>MRGCLRLALLCALPWLLLAASPGHPAKSPRQPPAPRRDPFDAARGADFDHVYSGVVNLSTENIYSFNYTSQPDQVTAVRVYVNSSSENLNYPVLVVVRQQKEVLSWQVPLLFQGLYQRSYNYQEVSRTLCPSEATNETGPLQQLIFVDVASMAPLGAQYKLLVTKLKHFQLRTNVAFHFTASPSQPQYFLYKFPKDVDSVIIKVVSEMAYPCSVVSVQNIMCPVYDLDHNVEFNGVYQSMTKKAAITLQKKDFPGEQFFVVFVIKPEDYACGGSFFIQEKENQTWNLQRKKNLEVTIVPSIKESVYVKSSLFSVFIFLSFYLGCLLVGFVHYLRFQRKSIDGSFGSNDGSGNMVASHPIAASTPEGSNYGTIDESSSSPGRQMSSSDGGPPGQSDTDSSVEESDFDTMPDIESDKNIIRTKMFLYLSDLSRKDRRIVSKKYKIYFWNIITIAVFYALPVIQLVITYQTVVNVTGNQDICYYNFLCAHPLGVLSAFNNILSNLGHVLLGFLFLLIVLRRDILHRRALEAKDIFAVEYGIPKHFGLFYAMGIALMMEGVLSACYHVCPNYSNFQFDTSFMYMIAGLCMLKLYQTRHPDINASAYSAYASFAVVIMVTVLGVVFGKNDVWFWVIFSAIHVLASLALSTQIYYMGRFKIDLGIFRRAAMVFYTDCIQQCSRPLYMDRMVLLVVGNLVNWSFALFGLIYRPRDFASYMLGIFICNLLLYLAFYIIMKLRSSEKVLPVPLFCIVATAVMWAAALYFFFQNLSSWEGTPAESREKNRECILLDFFDDHDIWHFLSATALFFSFLVLLTLDDDLDVVRRDQIPVFENLYFQGDYKDDDDKHHHHHHHH[2x]

Two mammalian homologs of systemic RNA interference defective protein 1 (SID-1) (SIDT1/2) are suggested to function as double-stranded RNA (dsRNA) transporters for extracellular dsRNA uptake or for release of incorporated dsRNA from lysosome to cytoplasm. Here, we determine the cryo-electron microscopy structures of human SIDT1, homodimer in a side-by-side arrangement, with two distinct conformations, the cholesterol-bound form and the unbound form. Our structures reveal that the membrane-spanning region of SIDT1 harbors conserved histidine and aspartate residues coordinating to putative zinc ion, in a structurally similar manner to alkaline ceramidases or adiponectin receptors that require zinc for ceramidase activity. We identify that SIDT1 has a ceramidase activity that is attenuated by cholesterol binding.

Although clear densities corresponding to dsRNA were not observed, the cryo-EM structures of hSIDT1 in the presence of 25 bp dsRNA at pH5.0 were interestingly converged to 2 classes; one class is essentially same as the structure in the absence of dsRNA and similarly binds to cholesterol, while the other class has different conformation of the transmembrane (TM) region with no cholesterol binding. In the cholesterol-unbound form, the transmembrane region undergoes a large conformational change while the extracellular region is well fitted to that of the cholesterol-bound form structure (RMSD of 0.3 Å for Cα atoms). In the cholesterol-unbound form, TM5 rotates about 25° and its cytoplasmic side greatly moves from inside the membrane spanning region to the dimer interface (14 Å shift of the Cα atom of Thr592), which resulted in the interaction with TM2 of the other protomer. TM6 which interacts with TM2 in the cholesterol-bound form is pushed out (15.6 Å shift of the Cα atom of Tyr605) by the TM5 rotational motion and its N-terminal region is partially disordered. Of note, despite the transmembrane region undergoes a large conformational change, the homodimer is maintained in the cholesterol-unbound form by the alternative interface in which TM5 displaces TM6 in the cholesterol-bound form. In the cholesterol-unbound form, no lipid-like density was observed between TM5 and TM6, which suggests that cholesterol stabilize the cholesterol-bound form structure through binding to the concave between TM5 and TM6. Interestingly, a tunnel is found to be formed in the transmembrane region in the cholesterol-unbound form structure by the conformational change in the transmembrane region. This tunnel is surrounded by TM4, TM5, TM9, TM10, and TM11 and penetrates the transmembrane region by passing through beside the zinc ion. TM8 is supposed to be located outside TM7 according to the weak density although TM8 is disordered in the cryo-EM map of the cholesterol-unbound form, which strongly indicates that TM8 do not intercept the tunnel.> GHHHHHHMIEWIIRRSVANRFLVLMGALFLSIWGTWTIINTPVDALPDLSDVQVIIKTSYPGQAPQIVENQVTYPLTTTMLSVPGAKTVRGFSQFGDSYVYVIFEDGTDPYWARSRVLEYLNQVQGKLPAGVSAELGPDATGVGWIYEYALVDRSGKHDLADLRSLQDWFLKYELKTIPDVAEVASVGGVVKEYQVVIDPQRLAQYGISLAEVKSALDASNQEAGGSSIELAEAEYMVRASGYLQTLDDFNHIVLKASENGVPVYLRDVAKVQIGPEMRRGIAELNGEGEVAGGVVILRSGKNAREVIAAVKDKLETLKSSLPEGVEIVTTYDRSQLIDRAIDNLSGKLLEEFIVVAVVCALFLWHVRSALVAIISLPLGLCIAFIVMHFQGLNANIMSLGGIAIAVGAMVDAAIVMIENAHKRLEEWQHQHPDATLDNKTRWQVITDASVEVGPALFISLLIITLSFIPIFTLEGQEGRLFGPLAFTKTYAMAGAALLAIVVIPILMGYWIRGKIPPESSNPLNRFLIRVYHPLLLKVLHWPKTTLLVAALSVLTVLWPLNKVGGEFLPQINEGDLLYMPSTLPGISAAEAASMLQKTDKLIMSVPEVARVFGKTGKAETATDSAPLEMVETTIQLKPQEQWRPGMTM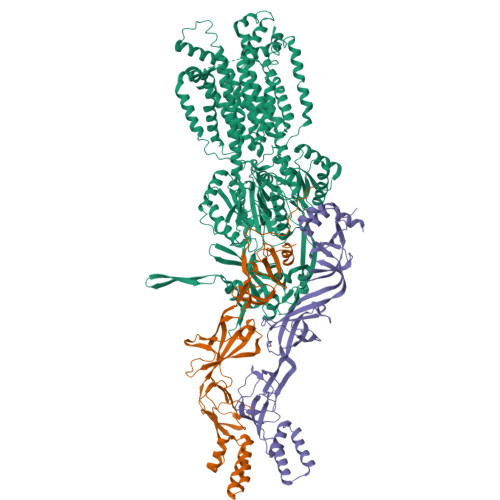DKIIEELDNTVRLPGLANLWVPPIRNRIDMLSTGIKSPIGIKVSGTVLADIDAMAEQIEEVARTVPGVASALAERLEGGRYINVEINREKAARYGMTVADVQLFVTSAVGGAMVGETVEGIARYPINLRYPQSWRDSPQALRQLPILTPMKQQITLADVADIKVSTGPSMLKTENARPTSWIYIDARDRDMVSVVHDLQKAIAEKVQLKPGTSVAFSGQFELLERANHKLKLMVPMTLMIIFVLLYLAFRRVGEALLIISSVPFALVGGIWLLWWMGFHLSVATGTGFIALAGVAAEFGVVMLMYLRHAIEAVPSLNNPQTFSEQKLDEALYHGAVLRVRPKAMTVAVIIAGLLPILWGTGAGSEVMSRIAAPMIGGMITAPLLSLFIIPAAYKLMWLHRHRVRK;>SASGVRIDPTQTQNLGVKTATVTRGPLTFAQSFPANVSYNEYQYAIVQARAAGFIDKVYPLTVGDKVQKGTPLLDLTIPDWVEAQSEYLLLRETGGTATQTEGILERLRLAGMPEADIRRLIATQKIQTRFTLKAPIDGVITAFDLRAGMNIAKDNVVAKIQGMDPVWVTAAIPESIAWLVKDASQFTLTVPARPDKTLTIRKWTLLPGVDAATRTLQLRLEVDNADEALKPGMNAWLQLNTASEPMLLIPSQALIDTGSEQRVITVDADGRFVPKRVAVFQASQGVTALRSGLAEGEKVVSSGLFLIDSEANISGALERMRSESATHAHHHHHHH[2x]>MRGSHHHHHHGSGATRIQIALKYDEKNKQFAILIIQLSNLSALLQQQDQKVNIRVAVLPCSESTTCLFRTRPLDASDTLVFNEVFWVSIAYPALHQKTLRVDVCTTDRSHLEECLGGAQISLAEV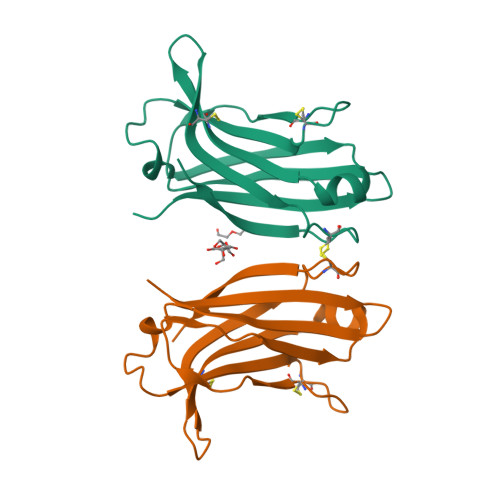CRSGERSTRWYNLLS[2x]> MRDLYRNTNTFMIRTPIFSIDNYYEFFRKDGESDKIKDRLLEICNNSVFREAILVSSKSLYSTIIDFCDGKEIKKFDYFLQSIYKYLIRMSMRPTPFGLFSGVDFGKYAEETVISYENDNFKKFARPDLEWIIKIVKELEDNHYKNLTFKINDSIFIKGERALLIHSTDKEDNNRIGEISIRATKPFMRTYDLAKDGIEYNKLKYILIDEYSIEDESKIDNFLKQLIEREFLISNLRPPLTVLDQFDYLINEVKKAEIEIPLVDELTEIKEKLKLYNETPVGAGEETYLELYKKMESVANVKNILQVDMKLNLRDKKINKKIISDVNDLMNILLDLSMSIENPEPFLSKYKQEFIEKYGQDREISLLEMLDNDIGIGPPMNYERPRNNRSLDVSVNELLDNNVRDYFMEKYFQALKTNSRNIAIRDDEIKNLELQKIDYENIPDSLEINLLVKNKSEDNLSDEFQYYIGPNLGSTSAGKSFGRFSHMMSEPKKFFEELDERNIELIDSEEYVTCEISYLPSEVRNANVTRNIHSSEYEMSLFTNGSKDNLYRIKLNDIYIGLENNTFYAKSKTLNKKLLLTINNMLNPQTAPNAIRFLNDISLDEKKLWYKFVWSDVYKDFSYIPAIKYKNFVIMPETWKMNKINMKINKKTEFNEFKNQFNDYRIKYGVPQYVYITFADNRILLNLDDEQCVKILYHECKNSFNEIILNSYEEEGVNIVKESHKDYICELVIPLTKIKQETISDKVSARMLSSDISSLSKER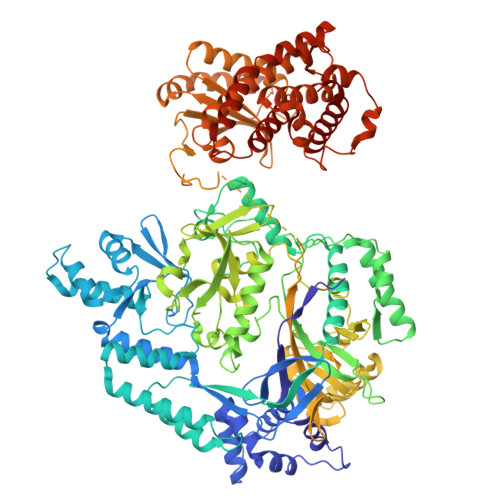VKDPFDEWLYIKLYGISSNVDDLIAYYISEFCNELVEEEIISKYFFMRYVDPEQHIRLRLNSSQEKLLMIYPKIREWLSMIRKKGLMTYFSIDSYDREIERYGGIELINIAEKVFFFDSIVTEDILRAKREGSFDFCDEIIGMISVVHYMESFGLPYAKQVEFLRSQVSSSEYREDFKQKRTEYMKLCNSNKDWEGLRESEEGNILIEILNKRRKIIEYYGNKVRENEEVSTDLSILDSIIHLNCNRMFGIDREFEKKVRALASHALYALKHFKS PTPN3 is a multidomain protein of 913 amino acids comprising a N-terminal FERM domain that determines subcellular localization, a central PDZ domain involved in protein-protein interactions, a short linker of 30-residues and a C-terminal protein tyrosine phosphatase (PTP) domain able to dephosphorylate protein substrates. The human protein tyrosine phosphatase non-receptor type 3 (PTPN3) is a phosphatase containing a PDZ (PSD-95/Dlg/ZO-1) domain that has been found to play both tumor-suppressive and tumor-promoting roles in various cancers, despite limited knowledge of its cellular partners and signaling functions. We solved the crystal structures of the complexes formed by PTPN3-PDZ with peptides comprising the PBMs of HPV 18 E6 (PBM-18E6) and of the cellular partner TACE (PBM-TACE). In all cases, the overall PDZ fold of PTPN3-PDZ is highly conserved, and the peptides bind in the conventional mode as an anti-parallel extension to the β2-strand.

Interestingly, viral proteins of oncoviruses, such as the capsid protein (HBc) of hepatitis B virus (HBV) and the E6 protein of high-risk human papillomaviruses types 16 and 18 (HPV16 and 18), possess PBMs that are able to interact with PTPN3. The PDZ-mediated interaction of E6 with PTPN3 results in the proteasomal degradation of the phosphatase. We previously obtained KD values of 26 μM, 29 μM, 53 μM and 37 μM for PBM-p38γ, PBM-HBc, PBM-16E6 and PBM-18E6, respectively, using the same methodology. All the complexes possess the classical bonding network of class I PDZ/PBM interactions (S/T-X-ΦCOOH). The C-terminal residues that exhibit well-defined electron density maps start from P-5 for PBM-TACE, P-6 for PBMs of HPVs or P-7 for PBM-HBc until P0 (see peptide sequences in Table 1). As expected, the C-terminal carboxylate in each peptide forms three H-bonds with the amide nitrogens of F521, G522 and F523 of the “GLGF motif” on PTPN3-PDZ. The PBM-18E6 valine at P0 (V0) is additionally bonded to the carbonyl of G519 on the α1-β1 loop and to the Nζ of K580 of the α2-helix through a molecule of water. At P-2, the S or T side chains form H-bonds with the Nε2 of H572 at the N-terminus of the α2-helix of PTPN3-PDZ, which is conserved in class I PDZ domains. In PBM-18E6, on the contrary, the side chain does not contact the PDZ domain. In all our PTPN3-PDZ/peptide complexes and in the previously reported PTPN4-PDZ/peptide complexes, the E side chain at P-3 forms a bifurcated H-bond with the amide nitrogen of N524 and with the side chain hydroxyl of S538 in the β3 strand. In all four PBMs (PBM-HBc, PBM-16E6 and PBM-18E6 and PBM-TACE), the long and positively charged side chains of R or K at P-4 form ionic bonds with the carboxylate oxygens of D573 at the N-terminus of the α2-helix in PTPN3-PDZ.

>[2x]GAMGSSTEDASQYYCDKNDNGDSYLVLIRITPDEDGKFGFNLKGGVDQKMPLVVSRINPESPADTCIPKLNEGDQIVLINGRDISEHTHDQVVMFIKASRESHSRELALVIRRR;>[2x]RQERLQRRRETQV> GSMSSESDAANTEPE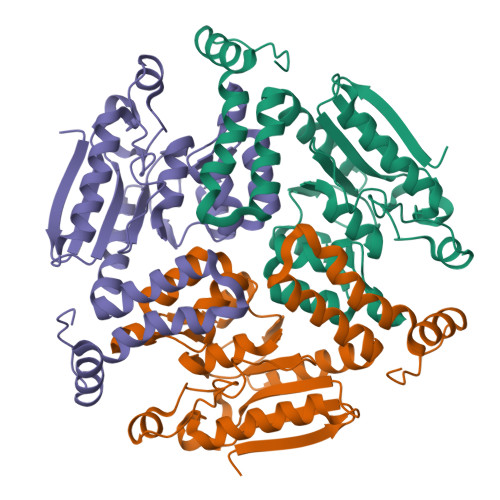VLVEQRDRILIITINRPKAKNAVNAAVSRGLADAMDQLDGDAGLSVAILTGGGGSFCAGMDLKAFARGENVVVEGRGLGFTERPPTKPLIAAVEGYALAGGTELALAADLIVAARDSAFGIPEVKRGLVAGGGGLLRLPERIPYAIAMELALTGDNLPAERAHELGLVNVLAEPGTALDAAIALAEKITANGPLAVVATKRIITESRGWSPDTMFAEQMKILVPVFTSNDAKEGAIAFAERRRPRWTGT> MDGTAAEPRPGAGSLQHAQPPPQPRKKRPEDFKFGKILGEGSFSTVVLARELATSREYAIKILEKRHIIKENKVPYVTRERDVMSRLD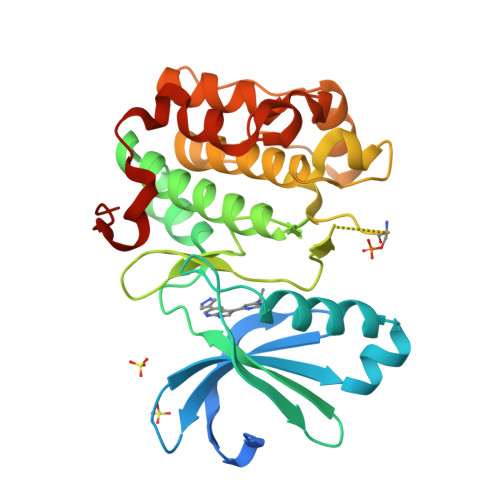HPFFVKLYFTFQDDEKLYFGLSYAKNGELLKYIRKIGSFDETCTRFYTAEIVSALEYLHGKGIIHRDLKPENILLNEDMHIQITDFGTAKVLSPESKQARANSFVGTAQYVSPELLTEKSACKSSDLWALGCIIYQLVAGLPPFRAGNEYLIFQKIIKLEYDFPEKFFPKARDLVEKLLVLDATKRLGCEEMEGYGPLKAHPFFESVTWENLHQQTPPKLT OCTANE-1,3,5,7-TETRACARBOXYLIC ACID | C12 H18 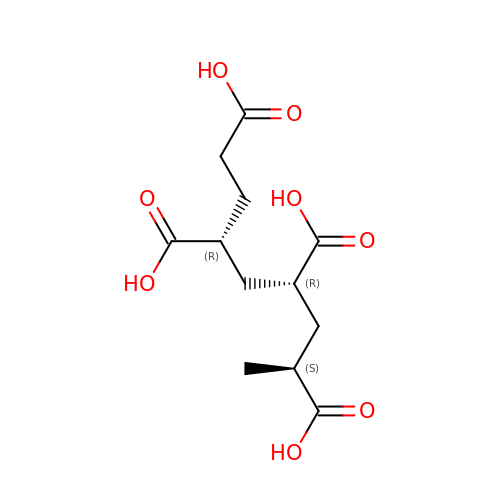O8 | UEYGDIASMOPQFG-XLPZGREQSA-N>[4x]RILPDSV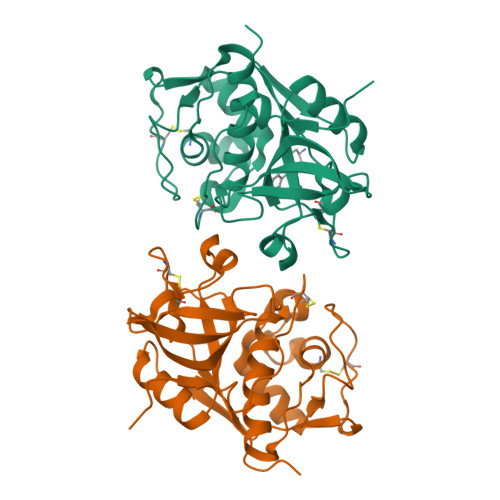DWREKGCVTEVKYQGSCGACWAFSAVGALEAQLKLKTGKLVSLSAQNLVDCSTEKYGNKGCNGGFMTTAFQYIIDNKGIDSDASYPYKAMDQKCQYDSKYRAATCSKYTELPYGREDVLKEAVANKGPVSVGVDARHPSFFLYRSGVYYEPSCTQNVNHGVLVVGYGDLNGKEYWLVKNSWGHNFGEEGYIRMARNKGNHCGIASFPSYPEIHHHHHH> XXXXXXXXXXXXLPAIAVIGDQSSGKSSVLEALSGVALPRGSGIVTRCPLVLKLKKLVNEDKWRGKVSYQDYEIEISDASEVEKEINKAQNAIAGEGMGISHELITLEISSRDVPDLTLIDLPGITRVAVGNQPADIGYKIKTLIKKYIQRQETISLVVVPSNVDIATTEALSMAQEVDPEGDRTIGILTKPDLVDKGTEDKVVDVVRNLVFHLKKGYMIVKCRGQQEIQDQLSLSEALQREKIFFENHPYFRDLL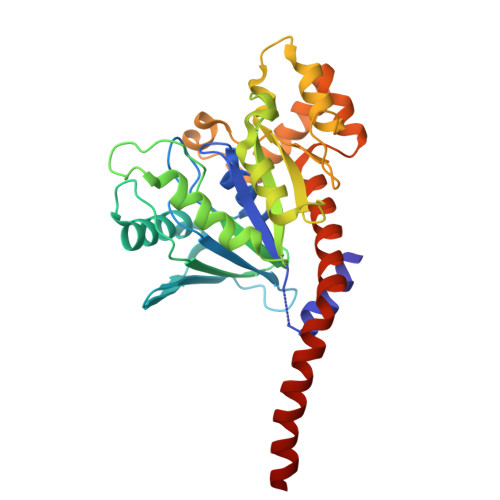EEGKATVPSLAEKLTSELITHISKSLPLLXXXXXXXXXXXXXXXXXX1-(4-aminophenyl)sulfonylguanidine 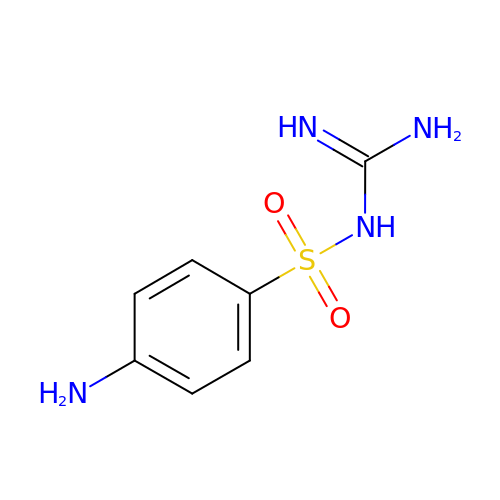| C7 H10 N4 O2 S | BRBKOPJOKNSWSG-UHFFFAOYSA-N> NDPESALNRAVGRVADTVASGPVNTEQIPALTAVETGHTSQVVPSDTMQTRHVINYHTRSESSIENFMGRAACVYIAQYATEKVNDELDRYTNWEITTRQVAQLRRKLEMFTYMRFDLEITFVITSSQRTSTTYASDSPPLTHQVMYVPPGGPIPKSYEDFAWQTSTNPSVFWTEGNAPPRMSIPFMSVGNAYCNFYDGWSHFSQSGVYGYTTLNNMGHLYFRHVNKSTAYPVNSVARVYFKPKHVKAWVPRAPRLCPYLKARNVNFNVQGVTESRNKITLDRSTHNPLANT;> SPTVEECGYSDRVRSITLGNSTITTQECANVVVGYGVWPTYLSDHEATAVDQPTQPDVATCRFYTLESVKWESSSAGWWWKFPEALSDMGLFGQNMQYHYLGRTGYTIHVQCNASKFHQGCLLVVCVPEAEMGAATTDHAFNHTKLSNIGQAMEFSAKKSTDQTGPQTAVHNAGMGVAVGNLTIFPHQWINLRTNNSATIVMPYINSVPMDNMYRHYNFTLMVIPFAKLEHSPQASTYVPITVTVAPMCAEYNGLRLAGHQ;> GLPTMNTPGSTQFLTSDDFQSPSAMPQFDVTPEIQIPGQVRNLMEIAEVDSVVPVNNTEGHVNSMEAYRIPVRPQTSSGEQVFGFQLQPGHDSVLKHTLLGEILNYYANWSGSMKLTFMYCGAAMATGKFLIAYSPPGAGVPGSRRDAMLGTHVIWDVGLQSSCVLCVPWISQTNYRYVTSDAYTDAGYITCWYQTSIVTPPDIPTTSTILCFVSACNDFSVRLLRDTPFITQQALFQ;> GAQVSTQKTGAHE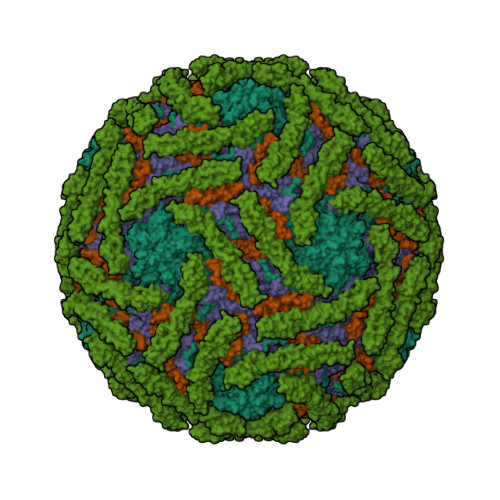TGLNASGNSIIHYTNINYYKDSASNSLNRQDFTQDPSKFTEPVKDVMIKTLPALN;> CNRSCEVPTRLNSASLKQPYITQNYFPVGTVVEYECRPGYRREPSLSPKLTCLQNLKWSTAVEFCKKKSCPNPGEIRNGQIDVPGGILFGATISFSCNTGYKLFGSTSSFCLISGSSVQWSDPLPECREIYCPAPPQIDNGIIQGERDHYGYRQSVTYACNKGFTMIGEHSIYCTVNNDEGEWSGPPPECRG>[6x]X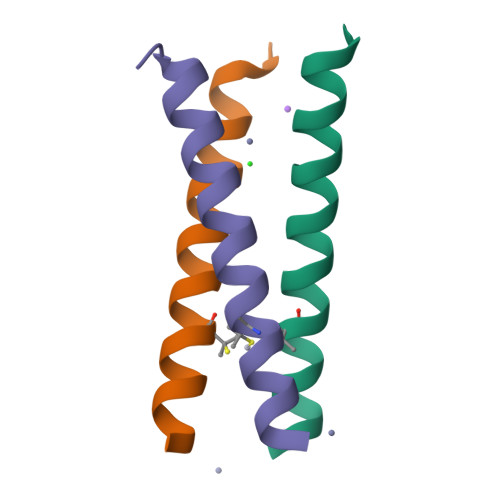EWEALEKKXAALESKLQALEKKHEALEHGX> KRPPLQEYVRKLLYKDLSKVTTEKVLRQMRKL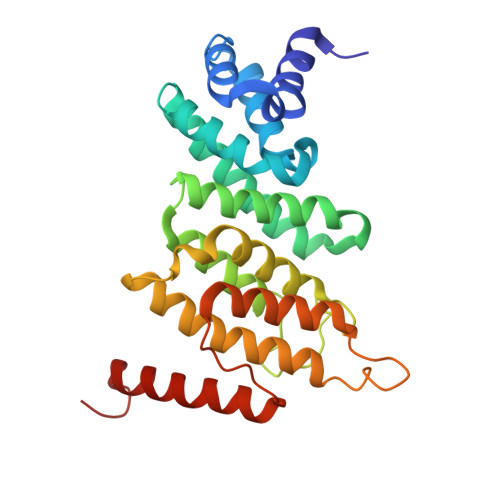PWQDQEVKDYVICCMINIWNVKYNSIHCVANLLAGLVLYQEDVGIHVVDGVLEDIRLGMEVNQPKFNQRRISSAKFLGELYNYRMVESAVIFRTLYSFTSFGVNPDGSPSSLDPPEHLFRIRLVCTILDTCGQYFDRGSSKRKLDCFLVYFQRYVWWKKSLEVWTKDHPFPIDIDYMISDTLELLRPKIKLCNSLEESIRQVQDLEREFLIKLGLVNDK>[3x]MFNMNINSPVRFVKETNRAKSPTRQSPGAAGYDLYSAYDYTIPPGERQLIKTDISMSMPKFCYGRIA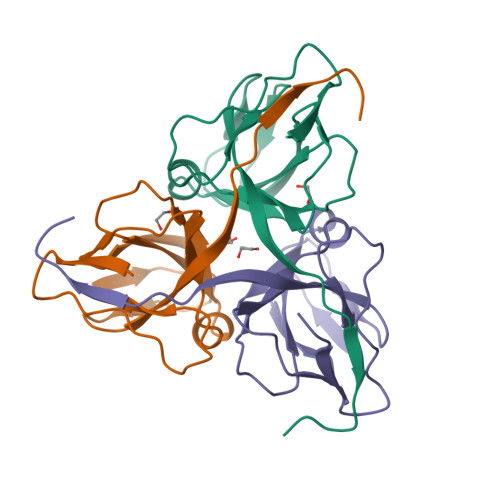PRSGLSLKGIDIGGGVIDEDYRGNIGVILINNGKCTFNVNTGDRIAQLIYQRIYYPELEEVQSLDSTNRGDQGFGSTGLR> SQKNYLELIKKVRERSNPDLVQMTKMYSETLSGSKLFENKSIEYSDVSIYIKESMKGVAPSYTMNSKVAANKVEAHLKKSHGNLVDFERQGSVMTNTHILKENDVDLVQITNKSSEFDHKGLEKALNNTSVLKTEEILNLKKHKENFSPYQGNQIDDLKYVRLKSELVLSSTYKTVDIEKENSIYVKVTEPERDIDVVTATYYKSVDFMKTNDKSRKGIQIYNKKTGKINDVDYPFLSIERIN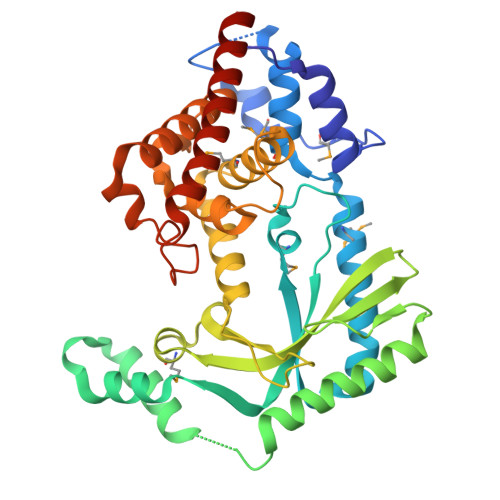VKDIISNRRLKNMIRFLKNIKYDCPHIENKGSIRSFHINAICYNIDVKKYEDLHYLDLVSILYQELTNIISNKSYRDNIKSVDGCEYIFEFDCAKKLIEIEFLSQELDSIIADLHNQSLLVG>[4x]MKAVAINGYGTVGKRVADAIAQQDDMKVIGVSKTRPDFEARMALKKGYDLYVAIPERVKLFEKAGIEVAGTVDDMLDEADIVIDCTPEGIGAKNLKMYKEKG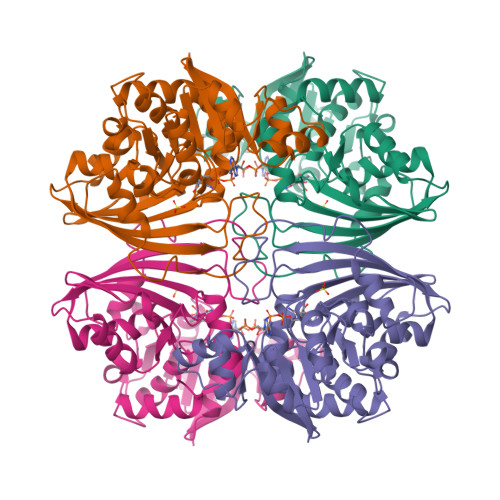IKAIFQGGEKHEDIGLSFNSLSNYEESYGKDYTRVVSCNTTGLCRTLKPLHDSFGIKKVRAVIVRRGADPAQVSKGPINAIIPNPPKLPSHHGPDVKTVLDINIDTMAVIVPTTLMHQHNVMVEVEETPTVDDIIDVFEDTPRVILISAEDGLTSTAEIMEYAKELGRSRNDLFEIPVWRESITVVDNEIYYMQAVHQESDIVPENVDAVRAILEMEEDKYKSINKTNKAMNILQ> MAGIAMKLATDREAAEGLGSHERAIKYLNQDYETLRNECLEAGALFQDPSFPALPSSLGFKELGPYSSKTRGIEWKRPTEICADPQFIIGGATRTDICQGALGDSWLLAAIASLTLNEEILARVVPLDQSFQENYAGIFHFQFWQYGEWVEVVVDDRLPTKDGELLFVHSAEGSEFWSALLEKAYAKINGCYEALSGGATTEGFEDFTGGIAEWYELRKPPPNLFKIIQKALEKGSLLGCSIDITSAADSEAVTYQKLVKGHAYSVTGAEEVESSGSLQKLIRIRNPWGQVEWTGKWNDNCPSWNTVDPEVRANLTERQEDGEFWMSFSDFLRHYSRLEICNLTPDTLTCDSYKKWKLTKMDGNWRRGSTAGGCRNYPNTFWMNPQYLIKLEEEDEDDEDGERGCTFLVGLIQKHRRRQRKMGEDMHTIGFGIYEVPEELTGQTNIHLSKNFFLTTRARERSDTFINLREVLNRFKLPPGEYVLVPSTFEPHKNGDFCIRVFSEKKADYQTVDDEIEANIEE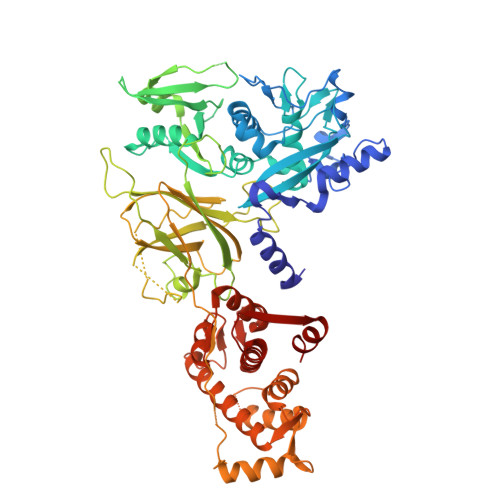IEANEEDIGDGFRRLFAQLAGEDAEISAFELQTILRRVLAKREDIKSDGFSIETCKIMVDMLDEDGSGKLGLKEFYILWTKIQKYQKIYREIDVDRSGTMNSYEMRKALEEAGFKLPCQLHQVIVARFADDELIIDFDNFVRCLVRLEILFKIFKQLDPENTGTIQLDLISWLSFSVL>MPFTYSIEATRNLATTERCIQDIRNAPVRNRSTQFQLAQQNMLAYTFGEVIPGFASAGINGMDYRDVIGRPVENAVTEGTHFFRDDFRVDSNAKAKVAGDIFEIVSSAVMWNCAARWNSLMVGEGWRSQPRYSRPTLSPSPRRQVAVLNLPRSFDWVSLLVPESQEVIEEFRAGLRKDGLGLPTSTPDLAVVVLPEEFQNDEMWREEIAGLTRPNQILLSGAYQRLQGRVQPGEISLAVAFARSLRSDRLYQPLYEANVMQLLLEGKLGAPKVEFEVHTLAPEGTNAFVTYEAASLYGLAEGRSAVHRAIRELYVPPTAADLARRFFAFLNERMEKVNGENLYFQSHHHHHH[2x]

SgrAI is a sequence specific type II restriction endonuclease that forms polymeric filaments with accelerated DNA cleavage activity and expanded DNA sequence specificity. Dimeric SgrAI binds both primary and secondary dsDNA recognition sequences in a 1:1 complex known as the DNA bound SgrAI dimer (or DBD). The SgrAI filament is a left-handed helix with approximately 4 DBD per turn. SgrAI is a divalent cation-dependent DNA endonuclease, and analogous to many DNA nucleases, likely uses the two divalent cations in a two-metal-ion cleavage mechanism.

The first structure, resolved to 3.3 Å, contains the active site mutation K242A, which inhibits DNA cleavage and leaves an intact phosphodiester bond at the cleavage site (hereafter known as the scissile phosphate [SP]). To make the SgrAIK242A/40-1/Mg2+ filamentous assembly, we incubated K242A SgrAI with a 40 bp DNA containing the primary sequence CACCGGTG (termed 40-1 DNA) in buffer containing MgCl2 and incubated for 30 min at room temperature prior to cryo-EM grid preparation. We observed filaments on cryo-EM grids and collected a dataset containing 3488 cryo-EM movies of the sample. Image processing using previously described workflows revealed a map resolved to 3.3 Å, which was sufficient for visualization of Mg2+ ions. The structure of SgrAIK242A/40-1/Mg2+ shows that the phosphodiester bond in the mutant form of the protein is intact. We were able to model 2 Mg2+ ions in the active site, in sites A and B, and the absence of the K242 side chain is evident. Mutation of this lysine results in greatly diminished rates of DNA cleavage. Consistent with these observations, our structure of SgrAI containing the K242A mutation showed no evidence of DNA cleavage, despite the presence of the biologically relevant and catalytically competent Mg2+ cofactor. The terminal amine of the K242A side chain remains within salt bridging distance with both the nucleophile and the SP, suggesting possible roles of the lysine side chain in catalysis, including positioning the nucleophile and SP for in-line attack, activation of the nucleophile, and stabilization of the transition state. Interestingly, the absence of the K242 side chain results in a shift in the position of the SP toward the space left by the missing side chain (Fig. 7B and in yellow in the middle panel), consistent with a role of the side chain in positioning the SP. Although we propose direct coordination by metal ion B to the O3′ and nonbridging oxygen of the SP prior to nucleophilic attack (second and third panels), these interactions are not observed in the SgrAIK242A/40-1/Mg2+ structure (the distance between the site B ion and the nonbridging oxygen is 4.2 Å, and between the site B ion and the O3′ is 3.1 Å). In addition, the distances between the carboxylate atoms of D188 and the Mg2+ ions in both sites A and B in the SgrAIK242A/40-1/Mg2+ structure are relatively long for direct coordination (2.9 and 2.8 Å, respectively).> MDGALINSVLYVSPRNGAHYFVELTEKHLLAFEMLNSMCLLENYDHVLLFLECQFGKSHNLAVIPFDIILVLF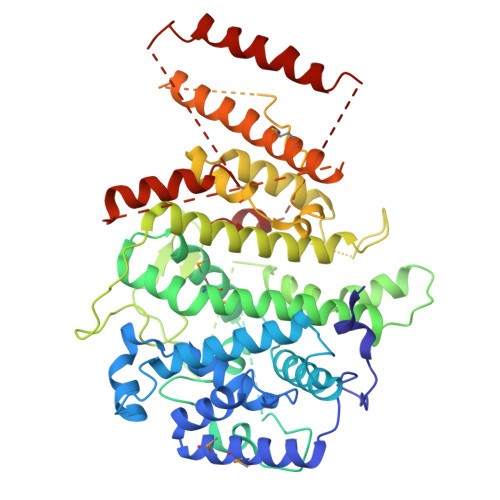TLSTLSEYYKEPILRANDPYNTSRETLSRRALKLLQKYLAILKEFDSEQYNLYDLELLRCQFFLAIDTLTPKKQKWGFDRFRRTKSESGVTYRQNASVDPELDQAKTFKNPYRSYISCLEQRNTILGNRLLNLKLNEPGEFINMILWTLSNSLQESTPLFLSSHEIWMPLLEILIDLFSCRQDYFIQHEVAQNVSKSLFVQRLSESPLAVFFESLNTRNFANRFSEYVFLNCDYKLPSDNYATPVHPVYNGENTIVDTYIPTIKCSPLYKSQKSLALRRKLIGSCFKLLLRVPDGHRLITPRIVADDVIQGISRTLASFNDILQFKKFFMTENLSQESYFIPLLAEGTLSEILKDTQECVVILTLVENLSDGVSFCNEVIGLVKSKCFAFTEQCSQASYEEAVLNIEKCDVCLLVLLRYLLHLIGTEAILDAKEQLEMLHAIEKNDSGRRQWAKALNLGNDPPLLYPIVSQMFGVHDKSVIIEXXXXXXXXXXXXXXXXXXXXXXXXXXXXXXXXXXXXXXXXXXXXXXXXXXX The Marasmius oreades agglutinin (MOA) is a 293 amino acid, homodimeric, histo-blood-group-B specific chimerolectin extracted from the fruiting bodies of the common fairy ring mushroom. Each MOA protomer is composed of two domains, accounting for the lectin’s sugar-binding and proteolytic functions, respectively. The proteolytic activity is associated to the C- terminal α+β dimerization domain, which closely resembles the consensus papain fold (r.m.s.d.: 2.2 Å), including the Cys/His catalytic dyad (Cys215, His257). In contrast to other known PLCPs, the proteolytic domain of MOA carries a binuclear calcium binding site.

The different orientations of Z-VAD-fmk were defined as ‘direct’ or ‘inverted’, depending on whether the VAD peptide was aligned with (‘direct’) or against (‘inverted’) the standard backbone orientation of a PLCP substrate. Consistent with known Z-VAD-fmk-bound complexes, the inhibitor molecule binds to the active site of MOA forming a thioether with the catalytic cysteine (Cys215). In the ‘direct’ orientation, the inhibitor molecule extends along the MOA dimerization interface, interacting with both protomers. The carbonyl group of the aspartate residue lies within hydrogen bonding distance of the backbone NH group of the catalytic cysteine (3.0 Å) and the indole NH of Trp208 (3.0 Å). The aspartate side chain of the inhibitor points away from the catalytic cleft, and forms a hydrogen bond with the backbone carbonyl oxygen of Ala256 (3.2 Å), which also engages in a hydrogen bonding interaction with the Asp backbone NH group (3.3 Å). The adjacent carbonyl group in the Ala-Asp peptide group interacts strongly with the solvent-exposed Ca2+ ion (2.3 Å), replacing a water molecule present in the calcium-bound structure of MOA. The side chain of the alanine moiety of the VAD peptidyl group snugly fits into a hydrophobic cavity lined by residues Leu247, Ala258 and Leu182# (‘#’ denotes a residue provided by the symmetry-related protomer). The carbonyl group of the Val-Ala peptide group contacts the backbone NH of Ala256 through a water-mediated interaction (Z-VAD-fmk-Ala3(O)/HOH: 2.4 Å). Based on the structural alignment with papain, Z-VAD-fmk occupies either the unprimed (S1-S3, ‘direct’ conformation) or the primed (S1’-S3’, ‘inverted’ conformation) subsites on the catalytic cleft of MOA. The S2 specificity pocket of MOA is defined by the P2 alanine side chain of Z-VAD-fmk.

> MSLRRGIYHIENAGVPSAIDLKDGSSSDGTPIVGWQFTPDTINWHQLWLAEPIPNVADTFTLCNLFSGTYMDLYNGSSEAGTAVNGWQGTAFTTNPHQLWTIKKSSDGTSYKIQNYGSKTFVDLVNGDSSDGAKIAGWTGTWDEGNPHQKWYFNRMSVSSAEAQAAIARNPHIHGTYRGYILDGEYLVLPNATFTQIWKDSGLPGSKWREQIYDCDDFAIAMKAAVGKWGADSWKANGFAIFCGVMLGVNKAGDAAHAYNFTLTKDHADIVFFEPQNGGYLNDIGYDSYMAFY>SNAMADTLLELPDDFSRVLAIVAHPDDIEFGAGPAVAQWTAQGREVAYLLVTRGEAGISDLEPAQCGPVREAEQRKAAAELGVHEVDFLDHYNDGTIEYGPGLRRDLARAVRRHRPELIVTFNHHDTWASGAWNTPDHRAVGLAALDAVADAANRWIFPELLDEGLEPWRAGKVAIAGSPHATHAVAVDDDSRDRAVRSLAAHDRYLGSLSDDPPQERAR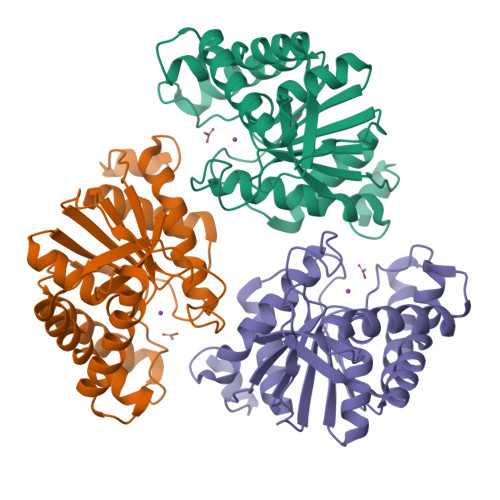FILGHLLAATAPRFGGRDGVAFQIVG[3x]> PISPIETVPVKLKPGMDGPKVKQWPLTEEKIKALVEICTEMEKEGKISKIGPENPYNTPVFAIKKKDSTKWRKLVDFRELNKRTQDFWEVQLGIPHPAGLKKKKSVTVLDVGDAYFSVPLDEDFRKYTAFTIPSINNETPGIRYQYNVLPQGWKGSPAIFQSSMTKILEPFRKQNPDIVIYQYMDDLYVGSDLEIGQHRTKIEELRQHLLRWGLYTPDKKHQKEPPFLWMGYELHPDKWTVQPIVLPEKDSWTVNDIQKLVGKLNWASQIYPGIKVRQLCKLLRGTKALTEVIPLTEEAELELAENR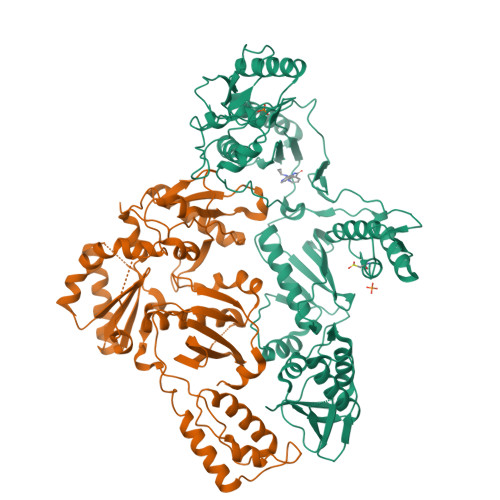EILKEPVHGVYYDPSKDLIAEIQKQGQGQWTYQIYQEPFKNLKTGKYARMRGAHTNDVKQLTEAVQKITTESIVIWGKTPKFKLPIQKETWETWWTEYWQATWIPEWEFVNTPPLVKLWYQLEKEPIVGAETFYVDGAANRETKLGKAGYVTNRGRQKVVTLTDTTNQKTELQAIYLALQDSGLEVNIVTDSQYALGIIQAQPDQSESELVNQIIEQLIKKEKVYLAWVPAHKGIGGNEQVDKLVSAGIRKVL;> PISPIETVPVKLKPGMDGPKVKQWPLTEEKIKALVEICTEMEKEGKISKIGPENPYNTPVFAIKKKDSTKWRKLVDFRELNKRTQDFWEVQLGIPHPAGLKKKKSVTVLDVGDAYFSVPLDEDFRKYTAFTIPSINNETPGIRYQYNVLPQGWKGSPAIFQSSMTKILEPFRKQNPDIVIYQYMDDLYVGSDLEIGQHRTKIEELRQHLLRWGLYTPDKKHQKEPPFLWMGYELHPDKWTVQPIVLPEKDSWTVNDIQKLVGKLNWASQIYPGIKVRQLCKLLRGTKALTEVIPLTEEAELELAENREILKEPVHGVYYDPSKDLIAEIQKQGQGQWTYQIYQEPFKNLKTGKYARMRGAHTNDVKQLTEAVQKITTESIVIWGKTPKFKLPIQKETWETWWTEYWQATWIPEWEFVNTPPLVKLWYQLEKEPIVGAETF>[104x]PLGHMPERFDAFICYCPSDIQFVQEMIRQLEQTNYRLKLCVSDRDVLPGTCVWSIASELIEKRCRRMVVVVSDDYLQSKECDFQTKFALSLSPGAHQKRLIPIKYKA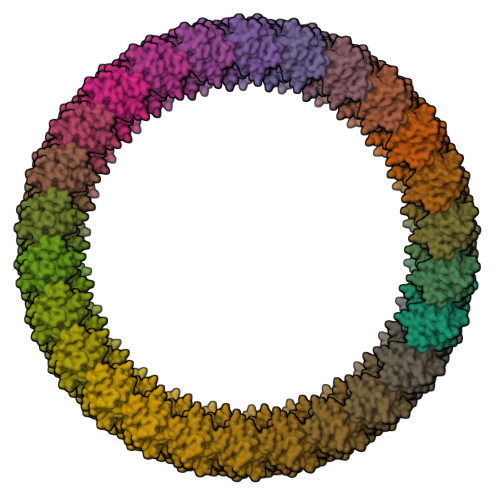MKKEFPSILRFITVCDYTNPCTKSWFWTRLAKALSLP3-{5-[AMINO(IMINIO)METHYL]-1H-INDOL-2-YL}-5-METHOXY-1,1'-BIPHENYL-2-OLATE 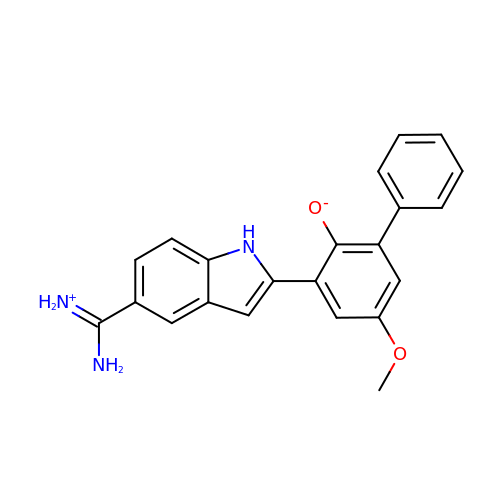| C22 H19 N3 O2 | MINVOLKUPZPDNX-UHFFFAOYSA-N>[2x]GSMGKPFFTRNPSELKGKFIHTKLRKSSRGFGFTVVGGDEPDEFLQIKSLVLDGPAALDGKMETGDVIVSVNDTCVLGHTHAQVVKIFQSIPIGASVDLELCRGYPLGSSAYGSVKAYTNFDAERDALNIETAIKTKGVDEVTIVNILTNRSNE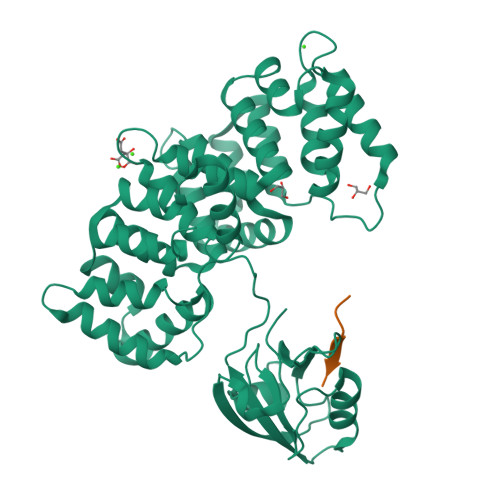QRQDIAFAYQRRTKKELASALKSALSGHLETVILGLLKTPAQYDASELKASMKGLGTDEDSLIEIICSRTNQELQEINRVYKEMYKTDLEKDIISDTSGDFRKLMVALAKGRRAEDGSVIDYELIDQDARDLYDAGVKRKGTDVPKWISIMTERSVPHLQKVFDRYKSYSPYDMLESIRKEVKGDLENAFLNLVQCIQNKPLYFADRLYDSMKGKGTRDKVLIRIMVSRSEVDMLKIRSEFKRKYGKSLYYYIQQDTKGDYQKALLYLCGGDD;>TDDSKPTRRETEV[2x]GIPC1 (GAIP interacting protein, C-terminus 1) and its two paralogs GIPC2 and GIPC3 are universal adaptor proteins that bind and regulate vesicular trafficking of many transmembrane proteins. GIPCs contribute to the endocytosis process by tethering the cargo proteins on endocytic vesicles to the motor protein myosin VI. GIPCs contain a central PDZ (PSD-95, Dlg and ZO-1) domain that mediates the interaction with the C-terminal PDZ-binding motif (PBM) in cargo proteins. The transmembrane receptor PlexinD1 contains a C-terminal ‘SEA’ motif that constitutes a PBM and interacts with GIPC1.

While full-length PlexinD1cyto failed to crystallize, we crystallized and determined the structures of a construct with the JM segment truncated (still referred to as PlexinD1cyto for simplicity), both in the apo-form (to 2.7 Å resolution) and in complex with GIPC1 (to 3.2 Å resolution). The structure of PlexinD1cyto in complex with GIPC1 is similar to apo-PlexinD1cyto, except in the C-terminal tail that binds GIPC1 (see details below). The entire PDZ-GH2 linker and GH2 domain of GIPC1 in the PlexinD1cyto/GIPC1 complex are invisible in the electron-density map. Binding of PlexinD1 to GIPC1 is expected to dislodge the GH2 domain from its autoinhibitory interaction with the PDZ domain, rendering the GH2 domain and the PDZ-GH2 linker conformationally flexible in relation to the GH1-PDZ module. The GH1 and PDZ domains of GIPC1 in the PlexinD1/GIPC1 complex are well structured and form the same domain-swapped dimer as apo-GIPC1. The two PlexinD1cyto molecules are placed at the opposite sides of the GIPC1 dimer and do not contact each other. In contrast, the tail segment in the PlexinD1cyto/GIPC1 complex adopts an ordered, extended conformation. As expected, the PBM interacts with the PDZ domain in GIPC1 in the typical PBM/PDZ-binding mode, where the PBM forms a short β-strand to pack in an anti-parallel fashion with strand β2 in the PDZ domain. In addition to these canonical PBM/PDZ interactions, GIPC1 makes extensive contacts with other residues in the C-terminal tail as well as the two preceding helices of PlexinD1, resulting in a large interface with the total buried surface area of 2072 Å2. Notably, Ile1918 and Y1919 in the tail of PlexinD1 plug into a hydrophobic pocket formed at the junction between the GH1 and PDZ domain.

> ELNRSQGIPFLEYKHFVTRTFFPKCSSLYEERYVLPSKTLNSQGGSPPQETHPLLGEWNIPEHCRPSMEEGISLFSSLLNNKHFLIVFVHALEQQKDFAVRDRCSLASLLTIALHGKLEYYTSIMKELLVDLIDASAAKNPKLMLRRTESVVEKMLTNWMSICMYGCLRETVGEPFFLLLCAIKQQINKGSIDAITGKARYTLNEEWLLRENIEAKPRNLNVSFQGCGMDSLSVRAMDTDTLTQVKEKILEAFCKNVPYSQWPRAEDVDLEWFASSTQSYVLRDLDDTSVVEDGRKKLNTLAHYKIPEGASLAMSLTDKKDSTLGRVKDLDTEKYFHLVLPTDELVEPKKSHRQSHRKKVLPEIYLTRLLSTKGTLQKFLDDLFKAILSIREDKPPLAVKYFFDFLEEQAEKRGISDPDTLHIWKTNSLPLRFWVNILKNPQFVFDIEKTDHIDACLSVIAQAFIDACSISDLQLGKDSPTNKLLYAKEIPEYRKTVQRYYKQIQDMTPLSEQEMNAHLAEESRKYQNEFNTNVAMAEIYKYAKRYRPQIMAALEANPTARRTQLQHKFEQVVALMENNIYECYSEA;> GPHMAALRPRLVFHTQLAHGSPTGRIEGFTNVKELYGKIAEAFRLPAAEVMFCTLNTHKVDMDKLLGGQIGLEDFIFAHVKGQRKEVEVFKSEEALGLTITDNGAGYAFIKRIKEGSVIDHIQLISVGDMIEAINGQSLLGCRHYEVARLLKELPRGRTFTLKLTEPRKAFDMISQRSAGGHPGSGPQLGTGRGTLRLRSRGPATVEDLPSAFEEKAIEKVDDLLESYMGIRDTELAATMVELGKDKRNPDELAEALDERLGDFAFPDEFVFDVWGAIGDAKVGRY> EVQDVNDSSWKEFVLESEVPVMVDFWAPWCGPSKLIAPVIDELAKEYSGKIAVYKLNTDEAPGIATQYNIRSIPTVLFFKNGERKESIIGAVPK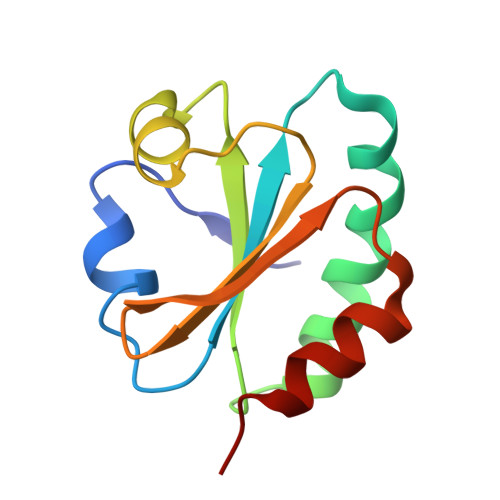STLTDSIEKYLS> SQLHYTVQEEQEHGTFVGNIAEDLGLDITKLSARGFQTVPNSRTPYLDLNLETGVLYVNEKIDREQICKQSPSCVLHLEVFLENPLELFQVEIEVLDINDNPPSFPEPDLTVEISESATPGTRFPLESAFDPDVGTNSLRDYEITPNSYFSLDVQTQGDGNRFAELVLEKPLDREQQAVHRYVLTAVDGGGGGGVGEGGGGGGGAGLPPQQQ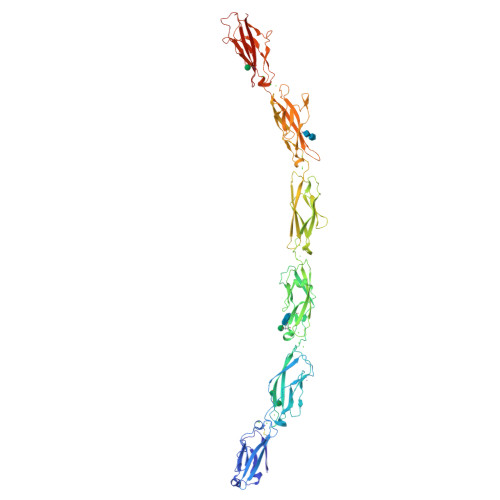RTGTALLTIRVLDSNDNVPAFDQPVYTVSLPENSPPGTLVIQLNATDPDEGQNGEVVYSFSSHISPRARELFGLSPRTGRLEVSGELDYEESPVYQVYVQAKDLGPNAVPAHCKVLVRVLDANDNAPEISFSTVKEAVSEGAAPGTVVALFSVTDRDSEENGQVQCELLGDVPFRLKSSFKNYYTIVTEAPLDREAGDSYTLTVVARDRGEPALSTSKSIQVQVSDVNDNAPRFSQPVYDVYVTENNVPGAYIYAVSATDRDEGANAQLAYSILECQIQGMSVFTYVSINSENGYLYALRSFDYEQLKDFSFQVEARDAGSPQALAGNATVNILIVDQNDNAPAIVAPLPGRNGTPAREVLPRSAEPGYLLTRVAAVDADDGENARLTYSIVRGNEMNLFRMDWRTGELRTARRVPAKRDPQRPYELVIEVRDHGQPPLSSTATLVVQLVDHHHHHH> GAHMKSTFKSEYPFEKRKAESERIADRFKNRIPVICEKAEKSDIPEIDKRKYLVPADLTVGQFVYVIRKRIMLPPEKAIFIFVN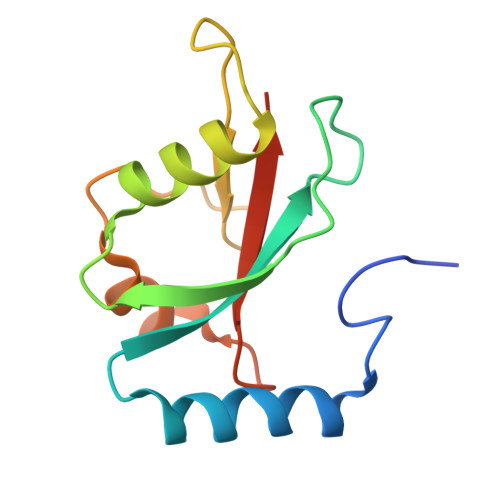DTLPPTAALMSAIYQEHKDKDGFLYVTYSGENTFG>GSMQPMLNIALRAARSAGELIFRSIERLDVISVNEKDAKDYVTEVDRAAEQTIVAALRKAYPTHAIMGEEGGLIEGSGEGADYLWVIDPLDGTTNFIHGVPHFAVSIACKYKGRLEHAVVLDPVRQEEFTASRGRGAALNGRRL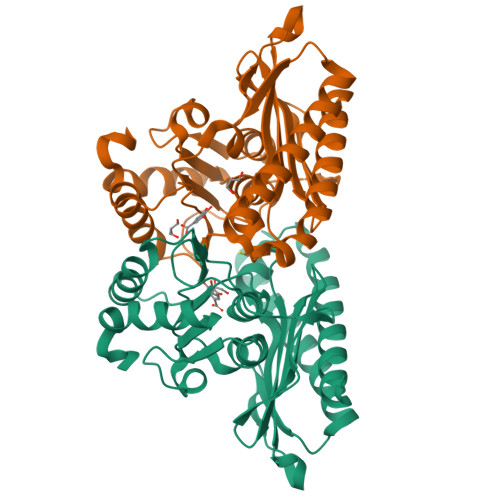RVSGRKSLEGALLGTGFPFRDNQIDNLDNYLNMFRSLVGQTAGIRRAGAASLDLAYVAAGRYDAFWEFGLSEWDMAAGALLVQEAGGLVSDFTGSHEFLEKGHIVAGNTKCFKALLTTIQPHLPPSLKR[4x]> MA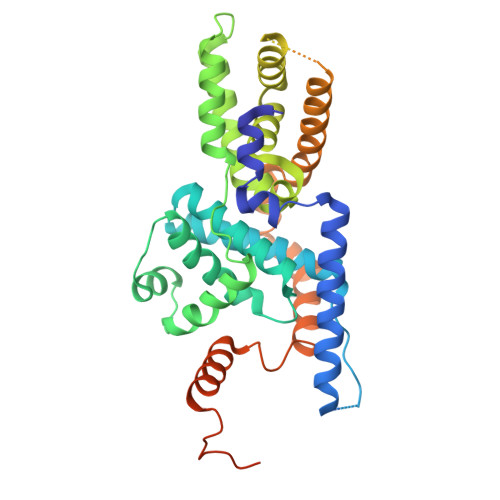STIASEDARYRQSSQYELWSFSPSQLASMREKTNAAARARITERLLSMPNPSNTASAPTSSANTPDPDGVSTPTLPEFLTPAEELLLVTFYTAELLRAGDHADMSDEIKATAATFFKRFYITNSIMTYPPQEMLLVALFFGCKAEGAFPSISDFAKTFGRERPEEILAGEFLLCQGIRFALDVKHPFRALRGAIMELSTLPDVEPARLVAAEQRAREILRFSPLITDAYFHFTPSQIMLAALSLADRGLAERLIQDTFHYVAPQPSSGTDTPATSGVETPSGASASISLHKRTASPSSGSLEDKAAVIGSHVRDKVLGTIEACRDMLSKELPERREHWNNKTVYKAQIQPIRKKLNKCRDPDRWNLVELQRIRREQASRKGFDSDDEGEGRTKGGSLEDDAAVFGVPKKKKQLEDPFGPPLAG> NLSELDRLLLEL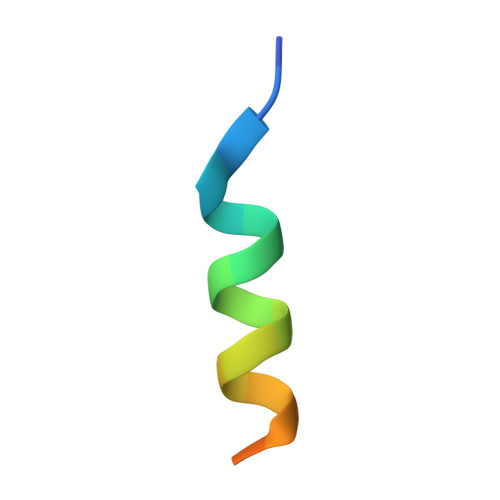NAVQHNPP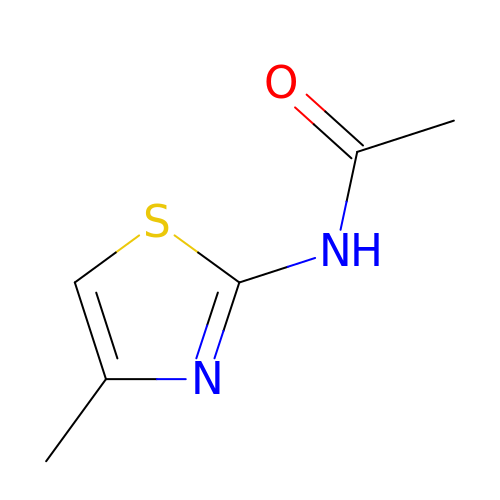~{N}-(4-methyl-1,3-thiazol-2-yl)ethanamide | C6 H8 N2 O S | DPDJXTANWGNJOE-UHFFFAOYSA-N(S)-2-METHYLMYRISTOYL-COENZYME 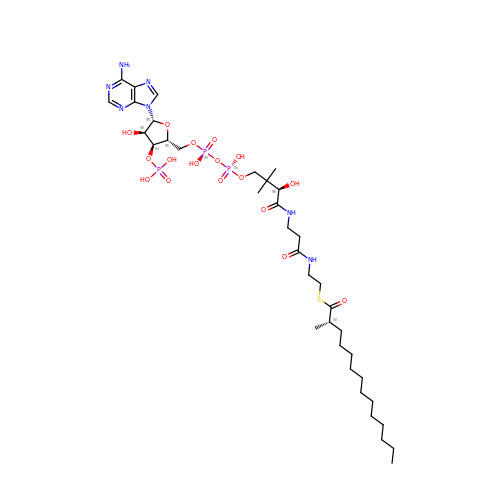A | C36 H64 N7 O17 P3 S | KJEFZXSIQKASDI-YFHVBOCQSA-N As the sole target of neutralizing antibodies, the virion surface protein Env encodes a glycan shield to restrict the antibody access to antigenically conserved sites. Small protein mimics of the CONEs are designed by epitope transplantation and used as immunogens to focus the antibody response. Here we focus our protein design efforts on four CONEs, including the structural elements of β sheet 12/13/22 (CONE 1), α2 helix (CONE 2), loop C (CONE 4), and loop E (CONE 5).

The C2S5 scaffold is built on a four-helix bundle from apolipoprotein E3. The two helixes used to display the CONE 2 residues were well matched to the α2 helix in terms of the Cα-Cβ orientations. For instance, a discontinuous three β-strand motif was grafted onto CONE 1 scaffolds, while the two helixes on the CONE 2 and scaffold 5 design (C2S5, a similar nomenclature is followed for all designed proteins) displayed the α2 helix-specific residues. Comparison with the Env trimer protein revealed a high degree of mimicry: within the epitope region, the Cα RMSDs between the designed proteins and Env were 0.42 Å (C2S5) and 0.34 Å (C4S3), respectively, suggesting that our CONE mimetics accurately display the Env residues. The electron density maps revealed that the side chains of the grafted residues were well positioned relative to the computational model. We selected the most stable designs (C1S1, C2S5, and C4S3) for immunization experiments and further structural analysis. The CONE 1, 2, and 4 proteins were monomeric in solution, while the C5S3 design displayed rapid exchange between monomeric and dimeric states. No HIV-specific antibodies were obtained after immunization with CONE 2 (α2 helix).

> MGHHHHHHGSENLYFQGSGQRWELALGRFWDYLRWVQTLSEQVQEELLSSQVETKLNKLMQRTMEELKAYKSELEEQLTPVAEETRARLSKELQAAQARLGADMEDVCGRLVQYRGEVQAMLGQSTEELRVRLATHLNKLRQRLLEDADDLQKRLAVYQ> MQGQQKESLESLFTKDSDPTVLDAAEQFAQWTLPTVLTRDISGMDGKRTSLHRDYQSTGAVLVNSAST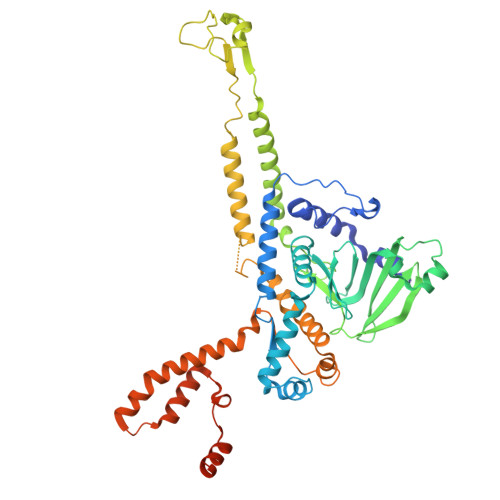KVTNALFPQGAPFFRFVDSPDMAAAVAELGINGTVQSQQSQIELSASSLVFSRDNYAASLRAVKLLMVTGNALEYFDEGTGRSHIYSVREYTVRRDGSGNILRVVLKERIAAMDLPQEFRSAHLGQKDDYDDVTLYTGICLEDNKFKIYQEVQQQQIGDASTYPIDECPYTVLVWNLVNGEHYGRGLVEDYAGDFARLSVLSQALTLYEVEAARLYNAVSAGAGIDVDAAQAAETGDYVQTSAAPGTNPGIWAVENGSDRKIMSLQSEISMIEQKLARAFMYAGNTRQGERVTAYEIRTNAQEAQNSLGDAYSILSDHWLRKRAYLYTVYQYPPMRAMFTLGATTIQILVGTASLNKAAQADRLLEASQSIQLVLPVLQGATKRTNPDAVVDFILDAFGVVSSKLMYTEEQLKQIQDQQDQQQADQQRNLELAQANPEVAGQQLGLIPS>[2x]MEEECRVLSIQSHVVRGYVGNRAATFPLQVLGFEVD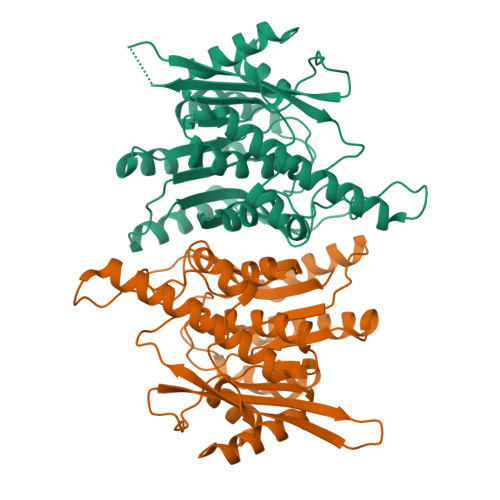AVNSVQFSNHTGYSHWKGQVLNSDELQELYDGLKLNHVNQYDYVLTGYTRDKSFLAMVVDIVQELKQQNPRLVYVCDPVMGDQRNGEGAMYVPDDLLPVYREKVVPVADIITPNQFEAELLTGRKIHSQEEALEVMDMLHSMGPDTVVITSSNLLSPRGSDYLMALGSQRTRAPDGSVVTQRIRMEMHKVDAVFVGTGDLFAAMLLAWTHKHPNNLKVACEKTVSAMHHVLQRTIKCAKAKSGEGVKPSPAQLELRMVQSKKDIESPEIVVQATVL N-(2-cyano-3-methyl-1H-indol-5-yl)butane-1-sulfonamide | C14 H17 N3 O2 S | 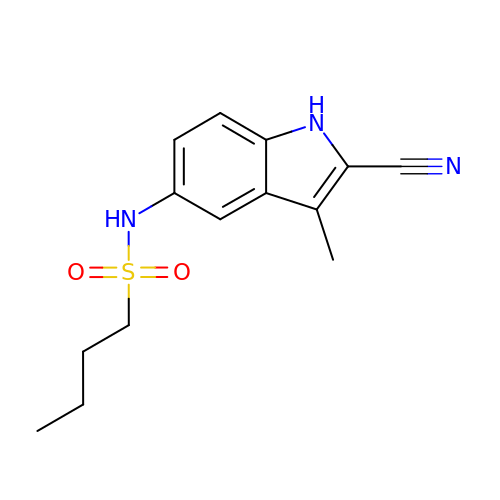NYTQGHHTLNYRJR-UHFFFAOYSA-N(2S,3R,4S,5S)-2-methyl-5-(1-phenyl-1H-1,2,3-triazol-4-yl)pyrrolidine-3,4-diol 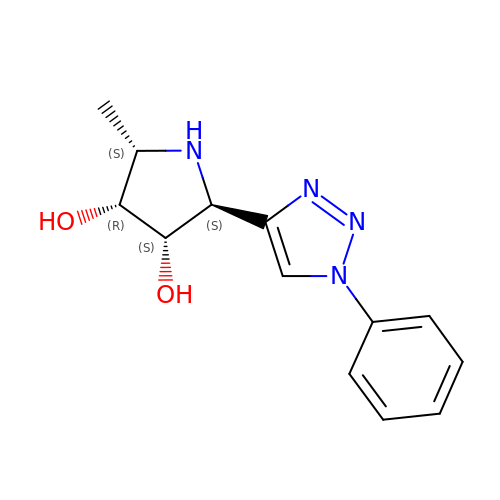| C13 H16 N4 O2 | HPPFSIKUULBMIZ-KNDHEWATSA-N>[3x]GSMEAVLNELVSVEDLLKFEKKFQSEKAAGSVSKSTQFEYAWCLVRSKYNDDIRKGIVLLEELLPKGSKEEQRDYVFYLAVGNYRLKEYEKALKYVRGLLQTEPQNNQAKELERLIDKAMKKDGL;>[4x]GSLDVGNAEVKLEEENRSLKADLQKLKDELASTKQKLEKAENQVLAMRKQSEGLTKEYDRLLEEHAKLSAAA

The outer mitochondrial membrane protein Fis1, known for its role in mitochondrial fission, has been reported to interact with the ER-resident protein Bap31. Fis1 is a single-pass integral membrane protein anchored in the OMM through its C-terminal transmembrane (TM) helix. Bap31, an alternative protein binding partner of Fis1, is an integral polytopic ER membrane protein. Fis1_ΔTM exhibited the six antiparallel α-helical repeat bundle structure known as the tetratricopeptide repeat (TPR)-like fold for protein binding.

The presence of both Fis1_ΔTM and Bap31_vDED in some crystals was confirmed by sodium dodecyl sulfate–polyacrylamide gel electrophoresis (SDS‒PAGE), and a crystal structure containing Fis1_ΔTM and Bap31_vDED (residues 168−233 + 234SAAA237; denoted as 168−233 + SAAA) was determined. The crystal structure contained three molecules of Fis1_ΔTM (chains A, B, and C) and four molecules of Bap31_vDED (two Bap31_vDED dimers, chains D−E and F−G) in an asymmetric unit. In the asymmetric unit of the crystal structure, two Fis1_ΔTM molecules (chains B and C) form a dimer with an extended α1 helix. Two individual coiled-coil (CC) dimers formed by four Bap31_vDED molecules (chains D−E and F−G) interact independently with two Fis1_ΔTM molecules (chains A and B) in the asymmetric unit. The remaining Fis1_ΔTM molecule (chain C) in the asymmetric unit did not interact with any Bap31_vDED molecule. The C-terminal region (from Asp224 to the C-terminal end) of the Bap31_vDED helix in the CC dimer bound to the convex side of Fis1_ΔTM, which consists mainly of α3 and α5 helices. The concave surface of Fis1 did not participate in the Fis1−Bap31 interaction. In particular, there is only one salt bridge and only one hydrogen bond between Fis1_ΔTM and Bap31_vDED: between the side chain of Lys64 (chain B, Fis1_ΔTM) and the side chain Asp224 (chain F, Bap31_vDED) form a salt bridge, and the side chain of Lys89 (chain B, Fis1_ΔTM) and the main chain carbonyl group of Ser234 (chain F, Ser234 is Gln234 in the wild type (WT) Bap31_vDED) form a hydrogen bond; when analyzed with chain B (Fis1_ΔTM) and chain F (Bap31_vDED). Since the buried surface area was only 273–361 Å2 (~3.4–5.3% and ~4.5% of the total surface areas of the Fis1_ΔTM and Bap31_vDED structures, respectively), the interaction between Fis1_ΔTM and BAP 31_vDED is likely very weak, explaining the impaired complex formation in the SEC experiment. Interestingly, although Fis1_ΔTM + Bap31_vDED crystals were grown under acidic conditions (pH 4.5), the C-terminus of Bap31_vDED had a defined helical structure.> MAFLDNPTIILAHIRQSHVTSDDTGMCEMVLIDHDVDLEKIHPPSMPGDSGSEIQGSNGETQGYVYAQSVDITSSWDFGIRRRSNTAQRLERLRKERQNQIKCKNIQWKERNSKQSAQELKSL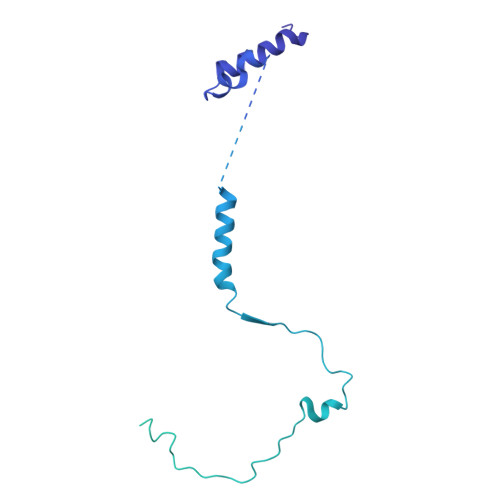FEKKSLKEKPPISGKQSILSVRLEQCPLQLNNPFNEYSKFDGKGHVGTTATKKIDVYLPLHSSQDRLLPMTVVTMASARVQDLIGLICWQYTSEGREPKLNDNVSAYCLHIAEDDGEVDTDFPPLDSNEPIHKFGFSTLALVEKYSSPGLTSKESLFVRINAAHGFSLIQVDNTKVTMKEILLKAVKRRKGSQKVSGPQYRLEKQSEPNVAVDLDSTLESQSAWEFCLVRENSSRADGVFEEDSQIDIATVQDMLSSHHYKSFKVSMIHRLRFTTDVQLGISGDKVEIDPVTNQKASTKFWIKQKPISIDSDLLCACDLAEEKSPSHAIFKLTYLSNHDYKHLYFESDAATVNEIVLKVNYILESRASTARADYFAQKQRKLNRRTSFSFQKEKKSGQQ> MADQAMTDQDQGAVTLYSGTAITDAKKNHPFSVKVGLAQVLRGGAIVEVSSVNQAKLAESAGACSVIVSDPVRSRGGVRRMPDPVLIKEVKRAVSVPVMARARVGHFVEAQILESLAVDYIDESEIISVADDDHFINKHNFRSPFICGCRDTGEALRRIREGAAMIRIQGDLTATGNIAETVKNVRSLMGEVRVLNNMDDDEVFTFAKKISAPYDLVAQTKQMGRVPVVQ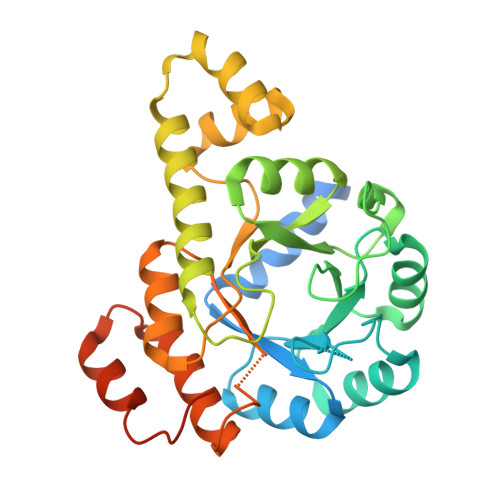FASGGITTPADAALMMQLGCDGVFVGSEVFDGPDPFKKLRSIVQAVQHYNDPHVLAEMSSGLENAMESLNVRGDRIQDFGQGSV The sodium channel NaV1.6 is widely expressed in neurons of the central and peripheral nervous systems, which plays a critical role in regulating neuronal excitability. Eukaryotic NaV channels are composed of a pore-forming α subunit and auxiliary β subunits. The four-domain α subunit exerts voltage sensing, gate opening, ion permeation, and inactivation. Meanwhile, one or two β subunits bind to the α subunit to regulate NaV channel kinetics and trafficking.

After processing, the final reconstruction map from the best class of ~41 k particles was refined to an overall resolution of 3.4 Å. Superposition of the Domain I ECLs of NaV1.6EM and NaV1.7 shows that the ECLI of NaV1.6EM lacks the short α2 helix, but instead forms an extended hairpin-like turn. Importantly, the ECLI of NaV1.6EM exhibits more N-linked glycosylation modification sites than NaV1.7; N308-linked glycosylation site appears to be unique for NaV1.6 based on the sequence alignment. Consistently, the signature fast inactivation gate, Ile-Phe-Met motif (IFM-motif), binds tightly to its receptor site adjacent to the intracellular activation gate, resulting in a non-conductive activation gate constricted by A411, L977, I1464, and I1765 from the four S6 helices, respectively. The van der Waals diameter of the activation gate is less than 6 Å, suggesting that the gate is functionally closed. Interestingly, two strong blobs of EM densities were observed in the SF of NaV1.6EM, which are deduced as potential Na+ binding sites because Na+ ions are the only major cations in the solutions throughout the purification processes. The upper site (namely Na1) closely engages E936 of the DEKA-locus and an additional acidic residue E939. The second blob of density is located inside the SF, namely the Na2 site, which is about ~5.3 Å away from the Na1 site. Thus, we hypothesize that the Na2 may represent the second step for sodium conductance, that is, after captured and partially dehydrated in Na1 site, at least partially-dehydrated Na+ can fit into the Na2 site which is going to enter the narrowest asymmetric constriction site of the SF.

> MAARLLAPPGPDSFKPFTPESLANIERRIAESKLKKPPKADGSHREDDEDSKPKPNSDLEAGKSLPFIYGDIPQGLVAVPLEDFDPYYLTQKTFVVLNRGKTLFRFSATPALYILSPFNLIRRIAIKILIHSVFSMIIMCTILTNCVFMTFSNPPDWSKNVEYTFTGIYTFESLVKIIARGFCIDGFTFLRDPWNWLDFSVIMMAYITEFVNLGNVSALRTFRVLRALKTISVIPGLKTIVGALIQSVKKLSDVMILTVFCLSVFALIGLQLFMGNLRNKCVVWPINFNESYLENGTKGFDWEEYINNKTNFYTVPGMLEPLLCGNSSDAGQCPEGYQCMKAGRNPNYGYTSFDTFSWAFLALFRLMTQDYWENLYQLTLRAAGKTYMIFFVLVIFVGSFYLVNLILAVVAMAYEEQNQATLEEAEQKEAEFKAMLEQLKKQQEEAQAAAMATSAGTVSEDAIEEEGEEGGGSPRSSSEISKLSSKSAKERRNRRKKRKQKELSEGEEKGDPEKVFKSESEDGMRRKAFRLPDNRIGRKFSIMNQSLLSIPGSPFLSRHNSKSSIFSFRGPGRFRDPGSENEFADDEHSTVEESEGRRDSLFIPIRARERRSSYSGYSGYSQGSRSSRIFPSLRRSVKRNSTVDCNGVVSLIGGPGSHIGGRLLPEATTEVEIKKKGPGSLLVSMDQLASYGRKDRINSIMSVVTNTLVEELEESQRKCPPCWYKFANTFLIWECHPYWIKLKEIVNLIVMDPFVDLAITICIVLNTLFMAMEHHPMTPQFEHVLAVGNLVFTGIFTAEMFLKLIAMDPYYYFQEGWNIFDGFIVSLSLMELSLADVEGLSVLRSFRLLRVFKLAKSWPTLNMLIKIIGNSVGALGNLTLVLAIIVFIFAVVGMQLFGKSYKECVCKINQDCELPRWHMHDFFHSFLIVFRVLCGEWIETMWDCMEVAGQAMCLIVFMMVMVIGNLVVLNLFLALLLSSFSADNLAATDDDGEMNNLQISVIRIKKGVAWTKLKVHAFMQAHFKQREADEVKPLDELYEKKANCIANHTGADIHRNGDFQKNGNGTTSGIGSSVEKYIIDEDHMSFINNPNLTVRVPIAVGESDFENLNTEDVSSESDPEGSKDKLDDTSSSEGSTIDIKPEVEEVPVEQPEEYLDPDACFTEGCVQRFKCCQVNIEEGLGKSWWILRKTCFLIVEHNWFETFIIFMILLSSGALAFEDIYIEQRKTIRTILEYADKVFTYIFILEMLLKWTAYGFVKFFTNAWCWLDFLIVAVSLVSLIANALGYSELGAIKSLRTLRALRPLRALSRFEGMRVVVNALVGAIPSIMNVLLVCLIFWLIFSIMGVNLFAGKYHYCFNETSEIRFEIEDVNNKTECEKLMEGNNTEIRWKNVKINFDNVGAGYLALLQVATFKGWMDIMYAAVDSRKPDEQPKYEDNIYMYIYFVIFIIFGSFFTLNLFIGVIIDNFNQQKKKFGGQDIFMTEEQKKYYNAMKKLGSKKPQKPIPRPLNKIQGIVFDFVTQQAFDIVIMMLICLNMVTMMVETDTQSKQMENILYWINLVFVIFFTCECVLKMFALRHYYFTIGWNIFDFVVVILSIVGMFLADIIEKYFVSPTLFRVIRLARIGRILRLIKGAKGIRTLLFALMMSLPALFNIGLLLFLVMFIFSIFGMSNFAYVKHEAGIDDMFNFETFGNSMICLFQITTSAGWDGLLLPILNRPPDCSLDKEHPGSGFKGDCGNPSVGIFFFVSYIIISFLIVVNMYIAIILENFSVATEESADPLSEDDFETFYEIWEKFDPDATQFIEYCKLADFADALEHPLRVPKPNTIELIAMDLPMVSGDRIHCLDILFAFTKRVLGDSGELDILRQQMEERFVASNPSKVSYEPITTTLRRKQEEVSAVVLQRAYRGHLARRGFICKKTTSNKLENGGTHREKKESTPSTASLPSYDSVTKPEKEKQQRAEEGRRERAKRQKEVRESKC;> MHRDAWLPRPAFSLTGLSLFFSLVPPGRSMEVTVPATLNVLNGSDARLPCTFNSCYTVNHKQFSLNWTYQECNNCSEEMFLQFRMKIINLKLERFQDRVEFSGNPSKYDVSVMLRNVQPEDEGIYNCYIMNPPDRHRGHGKIHLQVLMEEPPERDSTVAVIVGASVGGFLAVVILVLMVVKCVRRKKEQKLSTDDLKTEEEGKTDGEGNPDDGAK;> MGRLLALVVGAALVSSACGGCVEVDSETEAVYGMTFKILCISCKRRSETNAETFTEWTFRQKGTEEFVKILRYENEVLQLEEDERFEGRVVWNGSRGTKDLQDLSIFITNVTYNHSGDYECHVYRLLFFENYEHNTSVVKKIHIEVVDKANRDMASIVSEIMMYVLIVVLTIWLVAEMIYCYKKIAAATETAAQENASEYLAITSESKENCTGVQVAE>EIGTGFPFDPHYVEVLGSRMHYVDVGPRDGTPVLFLHGNPTSSYLWRNIIPHVAPSHRCIAPDLIGMGKSDKPDLDYRFDDHVRYLDAFIEALGLEEVVLVIHDWGSALGFHWAKRNPERVKGIAFMEFIRPIPTWDEWPEFARELFQAFRTPDVGRELIIDQNAFIEGILPKFVVRPLTEVEMDHYREPFLKPVWREPLWRFPNELPIAGEPANIWALVEAYMNWLHQSPVPKLLFWGTPGVLIPPAEAARLAESLPNLKTVFIGPGLHYLQEDNPDLIGSEIARWLPAL[2x]

Haloalkane dehalogenases (HLDs; EC 3.8.1.5) are α/β-hydrolases that catalyze the hydrolytic cleavage of the carbon–halogen bond in diverse halogenated aliphatic hydrocarbons via SN2 nucleophilic substitution. Structurally, HLDs consist of a canonical α/β-hydrolase fold, which is composed of a central eight-stranded β-sheet domain surrounded by several α-helices (i.e. αβα sandwich architecture). In all HLDs, the active site is positioned in a hydrophobic pocket buried between the α/β-fold core and the cap domain, and this catalytic center is connected with the bulk solvent via a main tunnel and a slot tunnel. After several iteration cycles, we obtained an 11-point DhaA mutant, hereafter referred to as DhaA115, with outstanding thermostability (Tm = 73.5 °C) and thermophilicity, as demonstrated by a substantial shift in the optimal catalytic temperature (Topt = 65 °C).

We obtained crystals that belonged to the space group P1211 and diffracted at 1.6 Å resolution. The final model contains two enzyme molecules per asymmetric unit and has good values for deviation from the ideal (root mean-square deviation on the Cα atoms of 0.3 Å; Fig. S1†), with R-factor and R-free values of 0.16 and 0.18 respectively. The overall topology of the secondary structure elements is very similar to that of the wild-type DhaA. However, specific backbone re-arrangements are observed, which encompass the L9, L10 and L14 loops and the α4 and α9 helices (Fig. 1 and S2†). Additionally, we unambiguously identified in the electron density map the presence of bis-tris propane (B3P), glycerol (GOL) and isothiocyanate (SCN) molecules, which were bound to the DhaA115 enzyme. The bis-tris propane and glycerol molecules are bound on the protein surface, the former being also involved in crystal-packing contacts. There are three SCN-binding sites per enzyme molecule; two of them are also located on the enzyme surface while the last one is deeply buried in the active site cavity (Fig. S1†). Analysis of the enzyme access tunnels and the active site cavity in DhaA115 revealed that the volumes of both the main and the slot access tunnels are greatly reduced, and that the enzyme active site is occluded. While partial closure of the main access tunnel was previously observed in several engineered DhaA variants, the simultaneous closure of both the main and the slot tunnels is a unique feature seen for the first time in DhaA115. This double-lock is enabled by: (i) the triplet of residues (L148, I172 and F176), coupled with the re-positioning of the α4 helix, that lock the main access tunnel and (ii) the structural re-arrangement of the L9 loop coupled with the re-positioning of the α9 helix, which lock the slot access tunnel.> MGSSHHHHHHSQDPNSMPDNTIQWDKDADGIVTLTMDDPSGSTNVMNEAYIESMGKAVDRLVAEKDSITGVVVASAKKTFFAGGDVKTMIQARPEDAGDVFNTVETIKRQLRTLETLGKPVVAAINGAALGGGLEIALACHHRIAADVKGSQLGLPAVTLGLLPGGGGVTRTVRMFGIQNAFVSVLAQGTRFKPAKAKEIGLVDELVATVEELVPAAKAWIKEELKANPD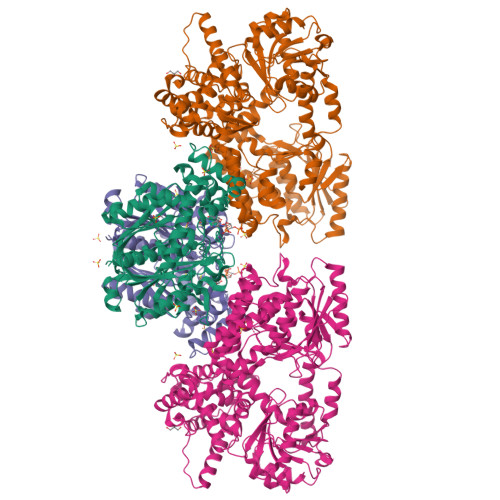GAGVQPWDKKGYKMPGGTPSSPGLAAILPSFPSNLRKQLKGAPMPAPRAILAAAVEGAQVDFDTASRIESRYFASLVTGQVAKNMMQAFFFDLQAINAGGSRPEGIGKTPIKRIGVLGAGMMGAGIAYVSAKAGYEVVLKDVSLEAAAKGKGYSEKLEAKALERGRTTQERSDALLARITPTADAADFKGVDFVIEAVFENQELKHKVFGEIEDIVEPNAILGSNTSTLPITGLATGVKRQEDFIGIHFFSPVDKMPLVEIIKGEKTSDEALARVFDYTLAIGKTPIVVNDSRGFFTSRVIGTFVNEALAMLGEGVEPASIEQAGSQAGYPAPPLQLSDELNLELMHKIAVATRKGVEDAGGTYQPHPAEAVVEKMIELGRSGRLKGAGFYEYADGKRSGLWPGLRETFKSGSSQPPLQDMIDRMLFAEALETQKCLDEGVLTSTADANIGSIMGIGFPPWTGGSAQFIVGYSGPAGTGKAAFVARARELAAAYGDRFLPPESLLS;> MSEEAFIYEAIRTPRGKQKNGSLHEVKPLSLVVGLIDELRKRHPDLDENLISDVILGCVSPVGDQGGDIARAAVLASGMPVTSGGVQLNRFCASGLEAVNTAAQKVRSGWDDLVLAGGVESMSRVPMGSDGGAMGLDPATNYDVMFVPQSIGADLIATIEGFSREDVDAYALRSQQKAAEAWSGGYFAKSVVPVRDQNGLLILDHDEHMRPDTTKEGLAKLKPAFEGLAALGGFDDVALQKYHWVEKINHVHTGGNSSGIVDGAALVMIGSAAAGKLQGLTPRARIVATATSGADPVIMLTGPTPATRKVLDRAGLTVDDIDLFELNEAFASVVLKFQKDLNIPDEKLNVNGGAIAMGHPLGATGAMILGTMVDELERRNARRALITLCIGGGMGVATIIERV>GMTISRNYDQEIKDTAGHKYAYNFDFDVMHPFMVRAFTPFFRPGNLLELGSFKGDFTSRLQEHFNDITCVEASEEAISHAQGRLKDGITYIHSRFEDAQLPRRYDNIVLTHVLEHIDDPVALLKRINDDWLAEGGRLFLVCPNANAVSRQIAVKMGIISHNSAVT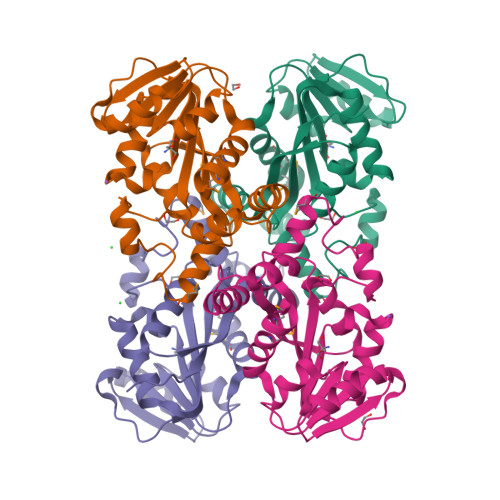EAEFAHGHRCTYALDTLERDASRAGLQVTYRSGIFFKALANFQWDQILQTDILSKEYLDGCYQLGQQYPDLCASIFLLCEKGINQ[4x]>[2x]SH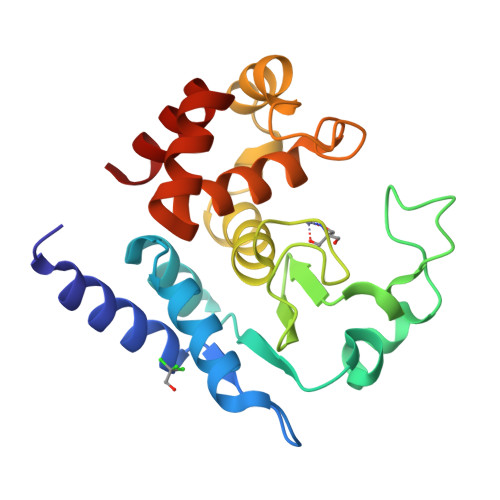MDSTTIQQNKDTLSQIVVFPTGNYDKNEANAMVNRLANIDGKYLNALKQNNLKIKLLSGKLTDEKEYAYLKGVVPKGWEGTGKTWDDVPGLGGSTVALRIGFSNKGKGHDAINLELHETAHAIDHIVLNDISKSAQFKQIFAKEGRSLGNVNYLGVYPEEFFAESFAYYYLNQDTNSKLKSACPQTYSFLQNLAK> SNQRMNDYSQPESQSDLAPKSSTIQPQPQPLLSKTPSMSLNLLSSSGPNRQVLPSEPSNFMTLMGQNGALLTVWALAKRNWLWAYPNIYSQDFGNIRNWKMEPGKHREYFRFVNQSLGTCVEAYGNGLIHDICSLDKLAQEFELLPTDSGAVVIKSVSQGRCVTYNPVSTTFYSTVTLSVCDGATEPSRDQTWYL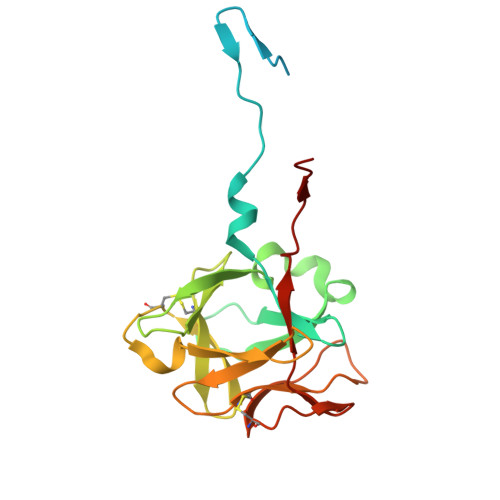APPVLEATAVN>MKLKALAAVALAAPLMVACGSTEKANEPFRLNGAGASFPAMLYSNWFTSFSKDTGNKVNYQAVGSGA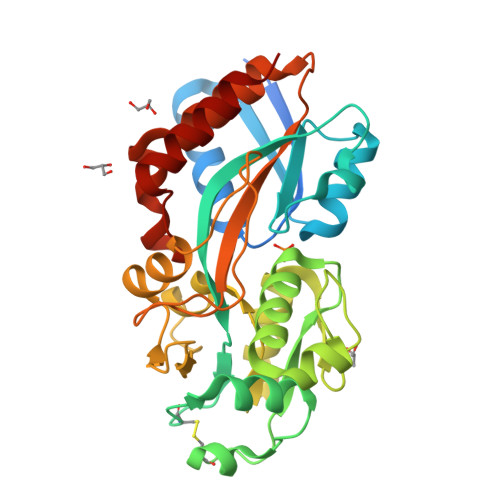GVRQFKAKTVDFGASDGAVKDSKQPAEGMVHIPMTGGAIVPAYNNPGCDLKMTQTELADVFLGKIDQWSHFGCEGGVIKTVHRSDGSGTTKGFTNSLSAFSPEWKKTVGTGKSVQWPVGVGGKGNSGVAAGIKLTPGSIGYVNYGYVQNDPALEQPALQNKAGNFVKASAETASAGLGEIVLDDQLRGADANPAGANAYPIVSLTWILAYPEYEKNEAVKEVLRYALTPTQQGKADSLGYVPLPESLRQKALAAVESLK[2x]> LPTAHEAIEAALADFVKVYNSKDAAGVASKYMDDAVIFPLDMARVDGRQN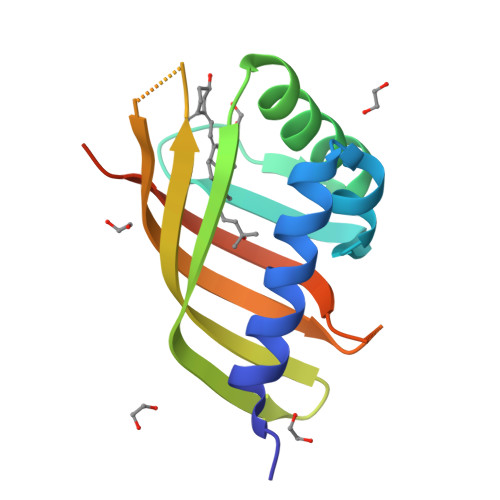IQKLWQGLMDMGVSEPKFTTLNVQESGDFAFESGSFSLKGPGKDSKLVDIAGIYVEVWRKGQDGGWKLYRTIANLDPARLEHHHHHH> ITYDKGIQTD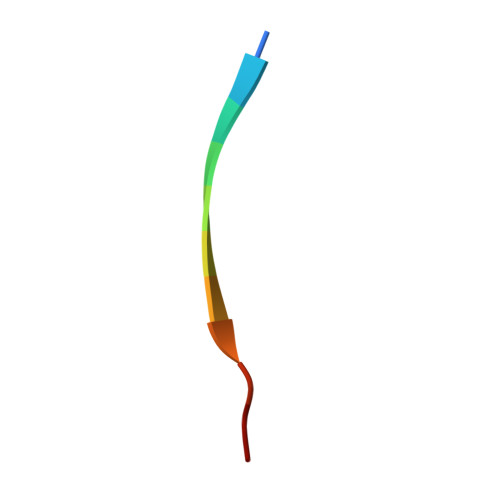Q> GGCUUAUCAA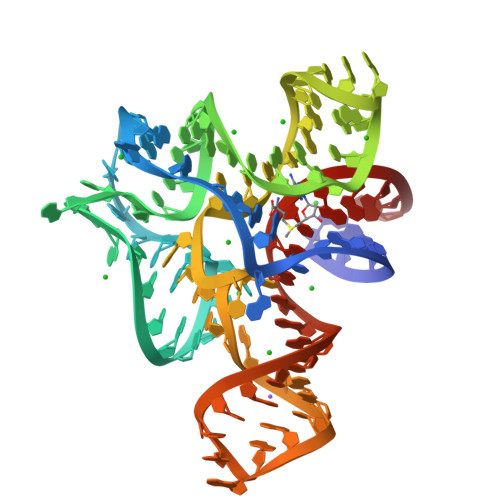GAGAGGGGGAGCGACUGGCGCGAAGAUCCCCGGCAACCAGAAAUGGUGCCAAUUCCUGCAGCGGAAACGUUGAAAGAUGAGCCG>[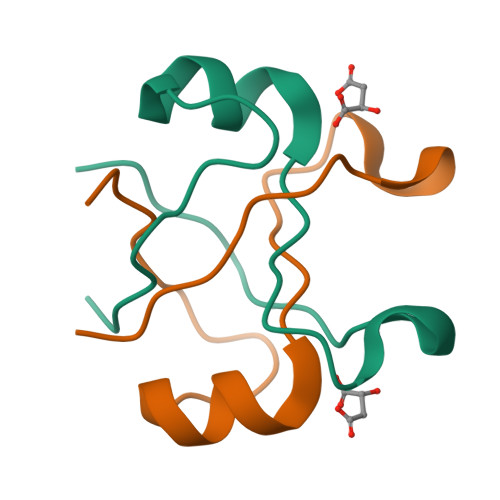4x]GPMPGKKVVARVAEARAEDVGKRVVRVDKAERAKVGVKVGDVVEVKKV>MGHHHHHHHHHSSGHIDDDDKHMDGLLEVVYGLLPENFPDPELAHDMVMWLAAKGYLPYDLERDDPELSVNIKGLTFHTPVGLAAGFDKNAEAPLNFCKMGFGFVEVGTITPKPQLGNPKPRIFRLAKDHAIINRCGFNSAGLDVVEPRLEKVSRDRWHDRLERHCVLGVNIGKNKDTVNAEDDIREGVKRVGRFADYLVINLSSPNTKGLRTLQQRDHLRSIITAAQSELEKLEERSRAQRERDGHSNPSEEEEAASSDSVTRKAEQFFPTQTGKRPLLFVKIAPDLTDEEKRDIADVALETGLDGLIVTNTTIQRPESLRSESKHETGGLSGRPLKAMSTKCVSDMYKMTNGQVAIIASGGIETGLDA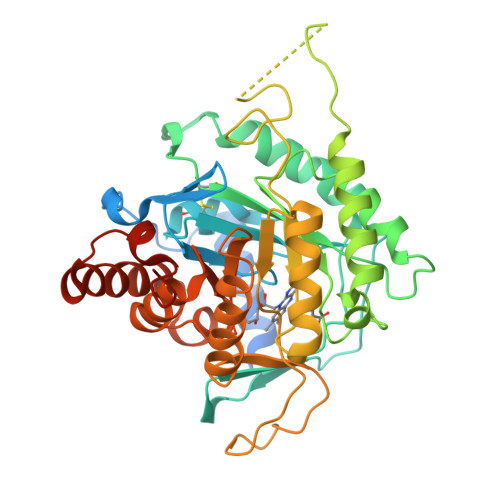YKRIRAGASAVEVYTSMIYRGPIVARRVKDELLNILNQAGIYNVQDAIGLDHRPPKKKRVRKPTFD[4x]> MARL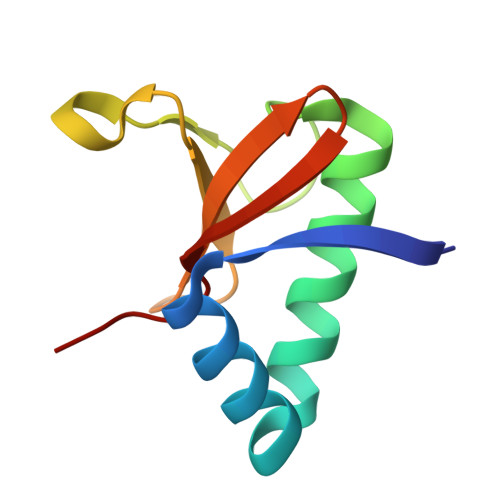NITFSPQAFEDYKYFQQNDKKMVKKINELLKSIDRNGALEGIGKPEKLKSNLTGYYSRRINHEHRLVYTVDDNHIKIASCKYHY>[4x]NKYFENVSKIKYEGPKSNNPYSFKFYNPEEVIDGKTMEEHLRFSIAYWHTFTADGTDQFGKATMQRPWNHYTDPMDIAKARVEAAFEFFDKINAPYFCFHDRDIAPEGDTLRETNKNLDTIVAMIKDYLKTSKTKVLWGTANLFSNPRFVHGASTSCNADVFAYSAAQVKKALEITKELGGENYVFWGGREGYETLLNTDMEFELDNFARFLHMAVDYAKEIGFEGQFLIEPKPKEPTKHQYDFDVANVL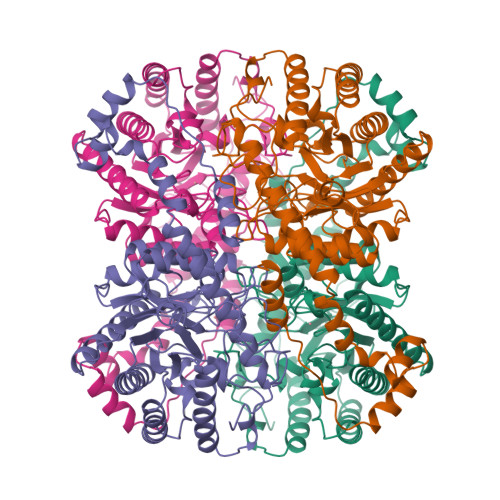AFLRKYDLDKYFKVNIEANHATLAFHDFQHELRYARINGVLGSIDANTGDMLLGWDTDQFPTDIRMTTLAMYEVIKMGGFDKGGLNFDAKVRRASFEPEDLFLGHIAGMDAFAKGFKVAYKLVKDRVFDKFIEERYASYKDGIGADIVSGKADFRSLEKYALERSQIVNKSGRQELLESILNQYLFAE> TLADQALHNNNVGPIIRAGDLVEPVIETAEIDNPGKEITVEDRRAYVRIAAEGELILTRKTLEEQLGRPFNMQELEINLASFAGQIQADEDQ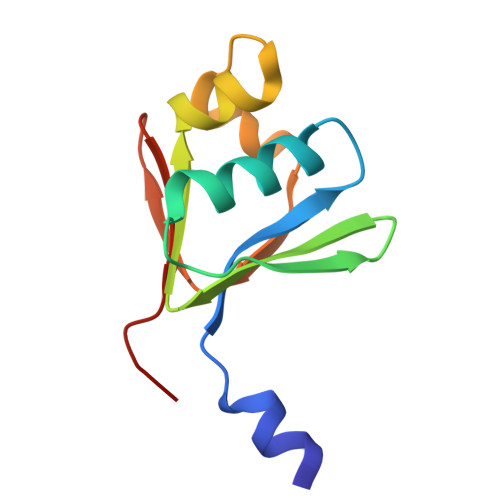IRFYFDKTM> MAGFWVGTAPLVAAGRRGRWPPQQLMLSAALRTLKHVLYYSRQCLMVSRNLGSVGYDPNEKTFDKILVANRGEIACRVIRTCKKMGIKTVAIHSDVDASSVHVKMADEAVCVGPAPTSKSYLNMDAIMEAIKKTRAQAVHPGYGFLSENKEFARCLAAEDVVFIGPDTHAIQA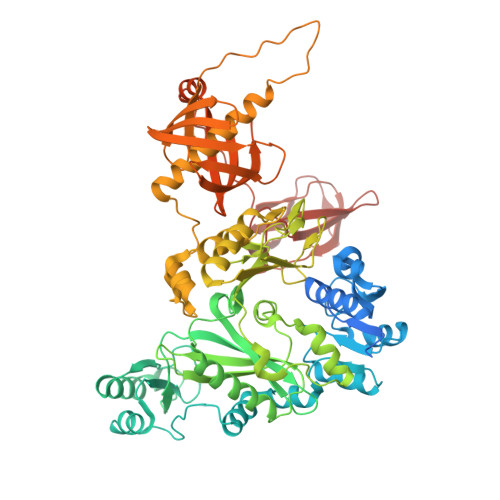MGDKIESKLLAKKAEVNTIPGFDGVVKDAEEAVRIAREIGYPVMIKASAGGGGKGMRIAWDDEETRDGFRLSSQEAASSFGDDRLLIEKFIDNPRHIEIQVLGDKHGNALWLNERECSIQRRNQKVVEEAPSIFLDAETRRAMGEQAVALARAVKYSSAGTVEFLVDSKKNFYFLEMNTRLQVEHPVTECITGLDLVQEMIRVAKGYPLRHKQADIRINGWAVECRVYAEDPYKSFGLPSIGRLSQYQEPLHLPGVRVDSGIQPGSDISIYYDPMISKLITYGSDRTEALKRMADALDNYVIRGVTHNIALLREVIINSRFVKGDISTKFLSDVYPDGFKGHMLTKSEKNQLLAIASSLFVAFQLRAQHFQENSRMPVIKPDIANWELSVKLHDKVHTVVASNNGSVFSVEVDGSKLNVTSTWNLASPLLSVSVDGTQRTVQCLSREAGGNMSIQFLGTVYKVNILTRLAAELNKFMLEKVTEDTSSVLRSPMPGVVVAVSVKPGDAVAEGQEICVIEAMKMQNSMTAGKTGTVKSVHCQAGDTVGEGDLLVELE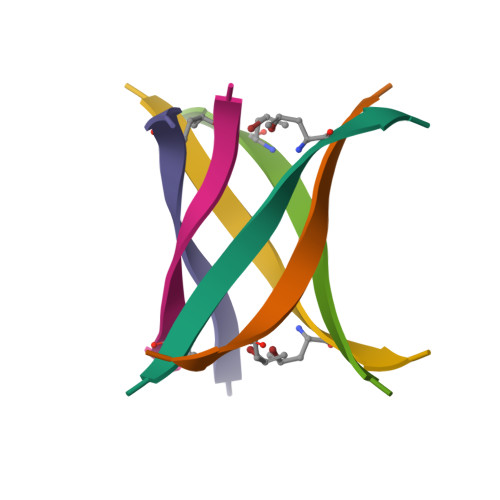>[2x]KVKVLGDXIEV> SGSNWRPQLLLLLSMQWSKEIIDVRYLNLLNLASQLKAGKGLTVVTAFLQGDPTSPDDKKKGEQVKARMDFDMNQVRLRGFAKTLVHSEDQVRGSMSTLVQSVGLGGLKPNTMLISWPVHEREEDMTEYNTFIEKVHAASINDMAIVVAKGIIDFPSAVFRMSGMIDVYWIVHDGGLCLLMGYLLKQHKVWRGCKLRVIGIAQESDNNVKMQEDLQKYVYQLRIDAKIMIVELADPEISKNAFERTLLMEERTMMMRDLQKVSGGGMSLSLPPANAPRAPSPLVTSERRANSKDSDEGTPTESEETTEKKSTSTD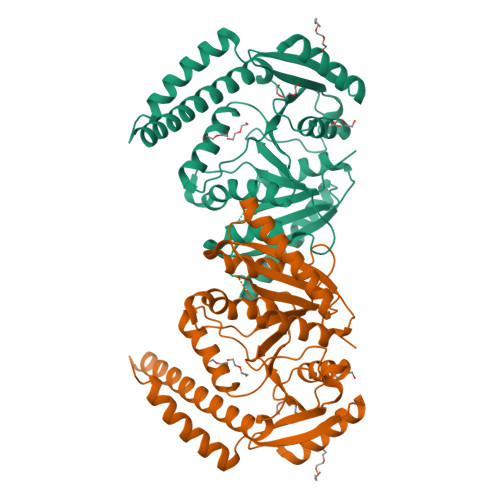NEQANQETKTKKERMKALDRSKVSKMHTAVRLNELLLQHSANSQLILLNLPKPPVHKDQQALDDYVHYLEVMTDKLNRVIFVRGTGKEVITESS>SNAMKISKVREENRGAKLTVNAKTAVVSENRSQEGILYNDPSRYGKSRKNDEDRDRYIESRLKSSGKLYRIFNEDKNKRETDELQWFLSEIVKKINRRNGLVLSDMLSVDDRAFEKAFEKYAELSYTNRRNKVSGSPAFETCGVDAATAERL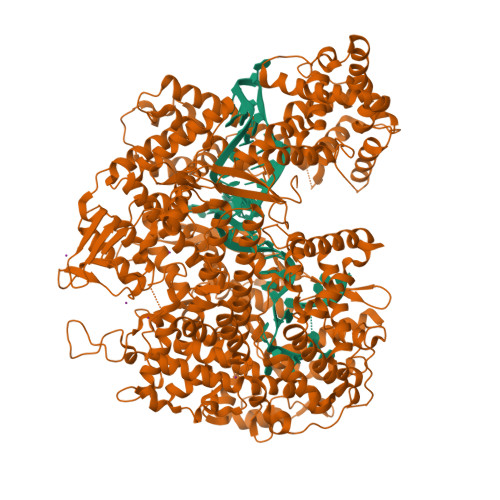KGIISETNFINRIKNNIDNKVSEDIIDRIIAKYLKKSLCRERVKRGLKKLLMNAFDLPYSDPDIDVQRDFIDYVLEDFYHVRAKSQVSRSIKNMNMPVQPEGDGKFAITVSKGGTESGNKRSAEKEAFKKFLSDYASLDERVRDDMLRRMRRLVVLYFYGSDDSKLSDVNEKFDVWEDHAARRVDNREFIKLPLENKLANGKTDKDAERIRKNTVKELYRNQNIGCYRQAVKAVEEDNNGRYFDDKMLNMFFIHRIEYGVEKIYANLKQVTEFKARTGYLSEKIWKDLINYISIKYIAMGKAVYNYAMDELNASDKKEIELGKISEEYLSGISSFDYELIKAEEMLQRETAVYVAFAARHLSSQTVELDSENSDFLLLKPKGTMDKNDKNKLASNNILNFLKDKETLRDTILQYFGGHSLWTDFPFDKYLAGGKDDVDFLTDLKDVIYSMRNDSFHYATENHNNGKWNKELISAMFEHETERMTVVMKDKFYSNNLPMFYKNDDLKKLLIDLYKDNVERASQVPSFNKVFVRKNFPALVRDKDNLGIELDLKADADKGENELKFYNALYYMFKEIYYNAFLNDKNVRERFITKATKVADNYDRNKERNLKDRIKSAGSDEKKKLREQLQNYIAENDFGQRIKNIVQVNPDYTLAQICQLIMTEYNQQNNGCMQKKSAARKDINKDSYQHYKMLLLVNLRKAFLEFIKENYAFVLKPYKHDLCDKADFVPDFAKYVKPYAGLISRVAGSSELQKWYIVSRFLSPAQANHMLGFLHSYKQYVWDIYRRASETGTEINHSIAEDKIAGVDITDVDAVIDLSVKLCGTISSEISDYFKDDEVYAEYISSYLDFEYDGGNYKDSLNRFCNSDAVNDQKVALYYDGEHPKLNRNIILSKLYGERRFLEKITDRVSRSDIVEYYKLKKETSQYQTKGIFDSEDEQKNIKKFQEMKNIVEFRDLMDYSEIADELQGQLINWIYLRERDLMNFQLGYHYACLNNDSNKQATYVTLDYQGKKNRKINGAILYQICAMYINGLPLYYVDKDSSEWTVSDGKESTGAKIGEFYRYAKSFENTSDCYASGLEIFENISEHDNITELRNYIEHFRYYSSFDRSFLGIYSEVFDRFFTYDLKYRKNVPTILYNILLQHFVNVRFEFVSGKKMIGIDKKDRKIAKEKECARITIREKNGVYSEQFTYKLKNGTVYVDARDKRYLQSIIRLLFYPEKVNMDEMIEVKEKKKPSDNNTGKGYSKRDRQQDRKEYDKYKEKKKKEGNFLSGMGGNINWDEINAQLKN[2x]C-reactive protein (CRP) is a pentameric protein of 115 kDa composed of five identical non-covalently associated pentraxin domains. The B-face binds to a range of ligands, with the canonical example being phosphocholine (PCh) head groups in lipids such as phosphatidylcholine. This is a calcium-dependent interaction, with each CRP monomer chelating two adjacent Ca2+ ions. The A-face modulates many effector functions of CRP, such as activation of the classical complement pathway, where binding of complement component C1q to CRP is mediated via predominantly electrostatic interactions between the Ca2+-containing globular head domain of C1q (gC1q) and the A-face of CRP.

Maps corresponding to pentameric CRP were solved with both C1 (no symmetry applied) and C5 symmetry. In all cases, applying C5 symmetry yielded maps of better resolution, corresponding to 3.2 – 3.3 Å. The increase in resolution upon map symmetrisation and high degree of similarity in the resulting maps and models strongly suggests that solution-phase CRP pentamers adopt C5 symmetry, which is reinforced by the low deviation in the angles between subunits in the C1-symmetrised pentameric models. Within the structures obtained by cryoEM, five intersubunit ionic bonds contribute to monomer-monomer interactions within the pentamer. These bonds form an ionic zipper from the A-face to the B-face of CRP. Upon the addition of PCh to the CRP pentamer, Lys123–Glu197 adopted an intermediate bond length of 4.6 Å. The addition of PCh resulted in an intermediate ionic bond length at this position. Hence, two factors that are known to prime CRP for complement activation, pH and PCh binding, appear to effect this bond. In all maps of pentameric and decameric CRP, clear density was present for two Ca2+ ions, and in conditions including PCh density for the ligand was visible and adopted similar conformations between the cryoEM derived models and those found in crystal structures.

>QTDMSRKAFVFPKESDTSYVSLKAPLTKPLKAFTVCLHFYTELSSTRGYSIFSYATKRQDNEILIFWSKDIGYSFTVGGSEILFEVPEVTVAPVHICTSWESASGIVEFWVDGKPRVRKSLKKGYTVGAEASIILGQEQDSFGGNFEGSQSLVGDIGNVNMWDFVLSPDEINTIYLGGPFSPNVLNWRALKYEVQGEVFTKPQLWP[5x]2-[[5-(6-methoxynaphthalen-2-yl)-3-oxidanyl-pyridin-2-yl]carbonylamino]ethanoic acid | C19 H16 N2 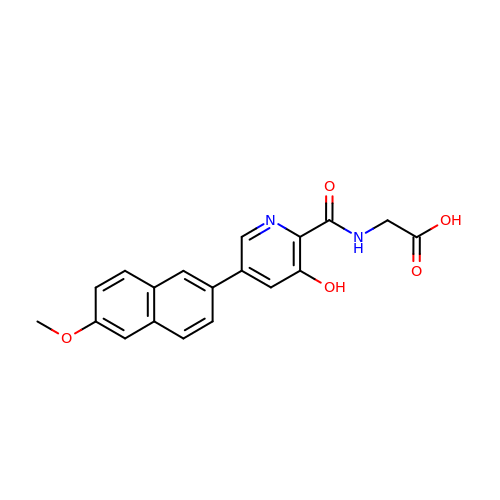O5 | PJNFXXUNCQIGBZ-UHFFFAOYSA-N> MSDQEAKPSTEDLGDKKEGEYIKLKVIGQDSSEIHFKVKMTTHLKKLKESY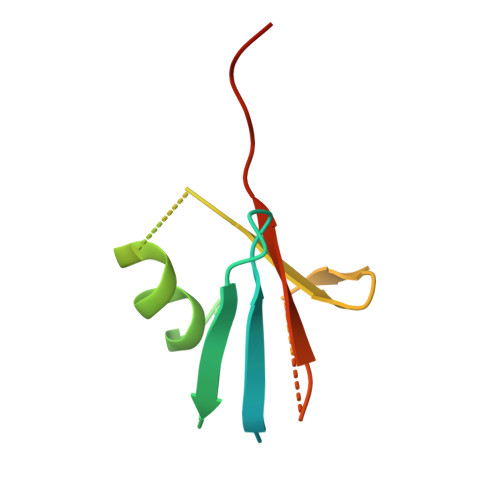CQRQGVPMNSLRFLFEGQRIADNHTPKELGMEEEDVIEVYQEQTGGHSTV> MSEPRFVHLRVHSDYSMIDGLAKTAPLVKKAAALGMPALAITDFTNLCGLVKFYGAGHGAGIKPIVGADFNVQCDLLGDELTHLTVLAANNTGYQNLTLLISKAYQRGYGAAGPIIDRDWLIELNEGLILLSGGRMGDVGRSLLRGNSALVDECVAFYEEHFPDRYFLELIRTGRPDEESYLHAAVELAEARGLPVVATNDVRFIDSSDFDAHEIRVAIHDGFTLDDPKRPRNYSPQQYMRSEEEMCELFADIPEALANTVEIAKRCNVTVRLGEYFLPQFPTGDMSTEDYLVKRAKEGLEERLAFLFPDEEERLKRRPEYDERLETELQVINQMGFPGYFLIVMEFIQWSKDNGVPVGPGRGSGAGSLVAYALKITDLDPLEFDLLFERFLNPERVSMPDFDVDFCMEKRDQVIEHVADMYGRDAVSQIITFGTMAAKAVIRDVGRVLGHPYGFVDRISKLIPPDPGMTLAKAFEAEPQLPEIYEADEEVKALIDMARKLEGVTRNAGKHAGGVVIAPTKITDFAPLYCDEEGKHPVTQFDKSDVEYAGLVKFDFLGLRTLTIINWALEMINKRRAKNGEPPLDIAAIPLDDKKSFDMLQRSETTAVFQLESRGMKDLIKRLQPDCFEDMIALVALFRPGPLQSGMVDNFIDRKHGREEISYPDVQWQHESLKPVLEPTYGIILYQEQVMQIAQVLSGYTLGGADMLRRAMGKKKPEEMAKQRSVFAEGAEKNGINAELAMKIFDLVEKFAGYGFNKSHSAAYALVSYQTLWLKAHYPAEFMAAVMTADMDNTEKVVGLVDECWRMGLKILPPDINSGLYHFHVNDDGEIVYGIGAIKGVGEGPIE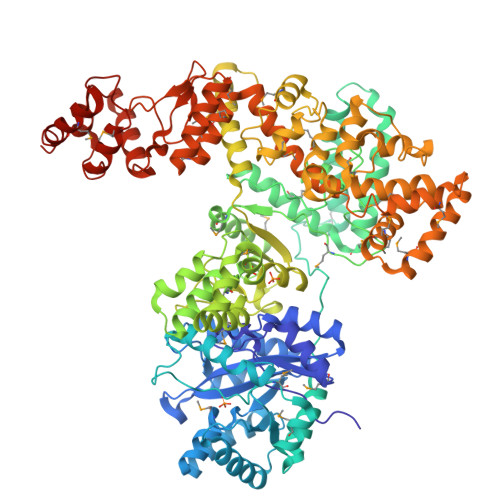AIIEARNKGGYFRELFDLCARTDTKKLNRRVLEKLIMSGAFDRLGPHRAALMNSLGDALKAADQHAKAEA>[2x]MMVISEKVRKALNDQLNREIYSSYLYLSMATYFDAEGFKGFAHWMKKQAQEEL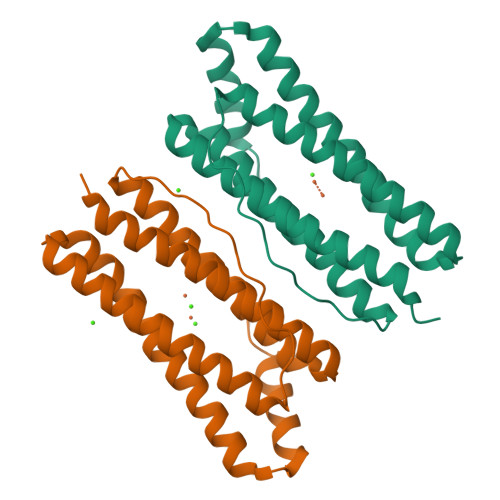THAMKFYEYIYERGGRVELEAIEKPPSNWNGIKDAFEAALKHEEFVTQSIYNILELASLALDHATVSFLKWFVDEQVEEEDQVREILDLLEKAFGQMSVIFQLDRYLGQRE>MRSKLLVPLVAAALCGAAITACAPPKAEQAKIAEIPDGTIDPAVWGKNYPEEYQTWKDTALPTPEGKSKYKKGNDGGKVYDKLSEYPFIALLFNGWGFGIEYNEPRGHVYMMKDQKEIDPSRLKGGGACLTCKTPYAPQLAQKQGVTYFSQSYADAVNQIPKEHQEMGVACIDCHNNKDMGLK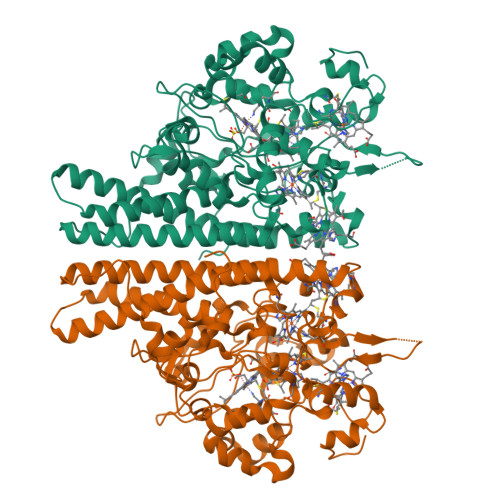ISRGFTLVKALDKMGVDQTKLTNQDKRSLVCAQCHVTYTIPKDANMKSQDVFFPWDESKWGKISIENIIKKMRSDKSYGEWTQAVTGFKMAYIRHPEFEMYSNQSVHWMAGVSCADCHMPYTKVGSKKISDHRIMSPLKNDFKGCKQCHSESSEWLKNQVITIQDRAASQYIRSGYALATVAKLFEMTHKQQAAGKQIDQKMYDQAKFYYEEGFYRNLFFGAENSIGFHNPTEAMRILGDATMYAGKADGLLRQALTKAGVDVPVKIDLELSKYTNNRGAKKLMFKPEQELKDPYGPQK[6x]> ANPLYQKHIISINDLSRDDLNLVLATAAKLKANPQPELLKHKVIASCFFEASTRTRLSFETSMHRLGASVVGF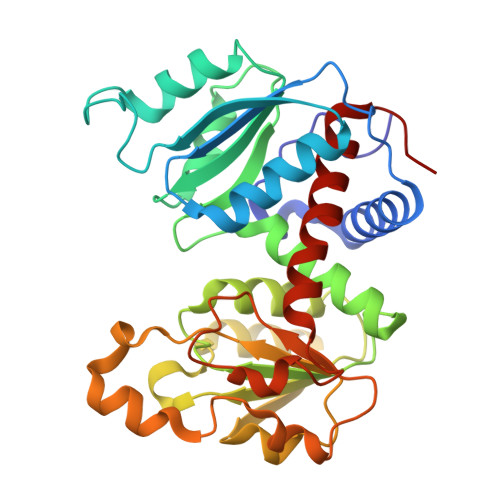SDSANTSLGKKGETLADTISVISTYVDAIVMRHPQEGAARLATEFSGNVPVLNAGDGSNQHPTQTLLDLFTIQETQGRLDNLHVAMVGDLKYGRTVHSLTQALAKFDGNRFYFIAPDALAMPQYILDMLDEKGIAWSLHSSIEEVMAEVDILYMTRVQKERLDPSEYANVKAQFVLRASDLHNAKANMKVLHPLPRVDEIATDVDKTPHAWYFQQAGNGIFARQALLALVLNRDLVL The CC chemokine receptor 7 (CCR7) balances immunity and tolerance by homeostatic trafficking of immune cells. Important homeostatic CC motif chemokine ligands are CCL19 and CCL21, which bind the CC chemokine receptor 7 (CCR7) to guide B cells, T cells, and antigen-presenting dendritic cells to lymph nodes throughout the body (Förster et al., 1999, Förster et al., 2008). The human CCR7 shares the seven transmembrane (TM1–TM7) helical fold of GPCRs where helices are connected by three intracellular (ICL) and three extracellular (ECL) loops. A short aliphatic helix (H8) anchors CCR7 in the cytoplasmic side of the membrane.

Here, we present the crystal structure of human CCR7 fused to the protein Sialidase NanA by using data up to 2.1 Å resolution. However, our structure showed Cmp2105 bound to a pocket at the intracellular part of CCR7 between the ends of TM1, TM2, TM3, and TM6 and the loop between TM7 and H8; this was similar to what was seen for CCR2-RA-[R] in CCR2 (Zheng et al., 2016), Vercirnon in CCR9 (Oswald et al., 2016), and Cmpd-15PA in the β2-adrenergic receptor (Liu et al., 2017). The two amino groups of Cmp2105 form hydrogen bonds with Asp942.40 indicating a central rolein positioning the central core motif. The sulfonyl group interacts with a conserved patch of residues at the turn between TM7 and H8 (Tyr3267.53, Gly3308.47, Val3318.48, Lys3328.49, and Phe3338.50). The substituents form interactions to several residues in TM2 (including hydrogen bonds to Thr912.37 and Thr932.39) and TM1 (mainly hydrophobic Val791.53, Thr821.56, and Phe861.60). They further bridge well-conserved residues including Arg1543.50 of the ERY motif in TM3 and Tyr3267.53 of the NPxxY motif in TM7, both part of the cytoplasmic cleft that opens upon GPCR activation (Scheerer et al., 2008). Cmp2105 stabilizes an inactive CCR7 conformation as evidenced by comparisons of our structure with the activated conformation of the CX3CL1-chemokine-bound viral US28 receptor (Burg et al., 2015) and the inactive conformation of the CCR2 receptor, with orthosteric and allosteric antagonists (Zheng et al., 2016). Our assignment to a deactivated CCR7 is further confirmed by a putative sodium ion in a conserved site between TM2, TM3, TM6, and TM7, which is known to negatively modulate activity in many GPCRs (Liu et al., 2012). Based on an overlay with the rhodopsin-Gi protein complex (Kang et al., 2018) and the rhodopsin-arrestin complex (Kang et al., 2015), the intracellular binding pocket spatially overlaps with the intracellular effector binding site of CCR7. The addition of this small molecule ligand results in a strong stabilizing effect of up to 20.1°C on CCR7 in thermofluor experiments.

> GPGSSLCSKKDVRNFKAWFLPIMYSIICFVGLLGNGLVVLTYIYFKRLKTMTDTYLLNLAVADILFLLTLPFWAYSAAKSWVFGVHFCKLIFAIYKMSFFSGMWLLLCISIDRYVAIVQAVSAHRHRARVLLISKLSCVGIWILATVLSIPELLYSDLQRSSSEQAMRCSLITEHVEAFITIQVAQMVIGFLVPLLAMSFCYLVIISKLHALTEKTDIFESGRNGNPNKDGIKSYRIPALLKTDKGTLIAGADERRLHSSDWGDIGMVIRRSEDNGKTWGDRVTITNLRDNPKASDPSIGSPVNIDMVLVQDPETKRIFSIYDMFPEGKGIFGMSSQKEEAYKKIDGKTYQILYREGEKGAYTIRENGTVYTPDGKATDYRVVVDPVKPAYSDKGDLYKGDQLLGNIYFTTNKTSPFRIAKDSYLWMSYSDDDGKTWSAPQDITPMVKADWMKFLGVGPGTGIVLRNGPHKGRILIPVYTTNNVSHLDGSQSSRVIYSDDHGKTWHAGEAVNDNRQVDGQKIHSSTMNNRRAQNTESTVVQLNNGDVKLFMRGLTGDLQVATSKDGGVTWEKDIKRYPQVKDVYVQMSAIHTMHEGKEYIILSNAGGPKRENGMVHLARVEENGELTWLKHNPIQKGEFAYNSLQELGNGEYGILYEHTEKGQNAYTLSFRKFNWEFLSKSKGHERNKAIKVIIAVVVVFIVFQLPYNGVVLAQTVANFNITSSTCELSKQLNIAYDVTYSLACVRCCVNPFLYAFIGVKFRNDLFKLFKDLGCLSGGRLEVLFQ>TSGEVKTSLKNAYSSAKRLSPKMEEEGEEEDYCTPGAFELERLFWKGSPQYTHVNEVWPKLYIGDEATALDRYRLQKAGFTHVLNAAHGRWNVDTGPDYYRDMDIQYHGVEADDLPTFDLSVFFYPAAAFIDRALSDDHSKILVHCVMGRSRSATLVLAYLMIHKDMTLVDAIQQVAKNRCVLPNRGFLKQL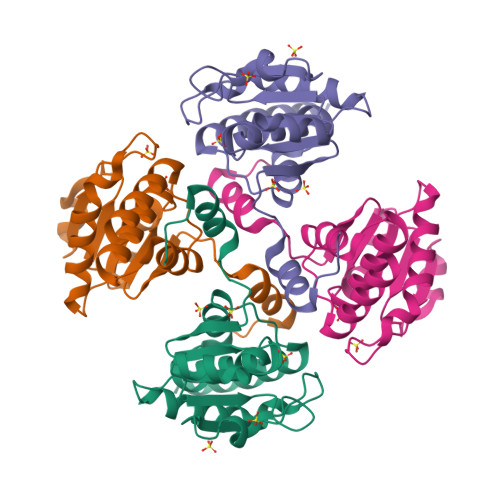RELDKQLVQQRRRSQRQDGEEEDGREL[2x]>[4x]MGHHHHHHMSNEGLCAVCGDNAACQHYGVRTCEGCKGFFKRTVQKNAKYVCLANKNCPVDKRRRNRCQ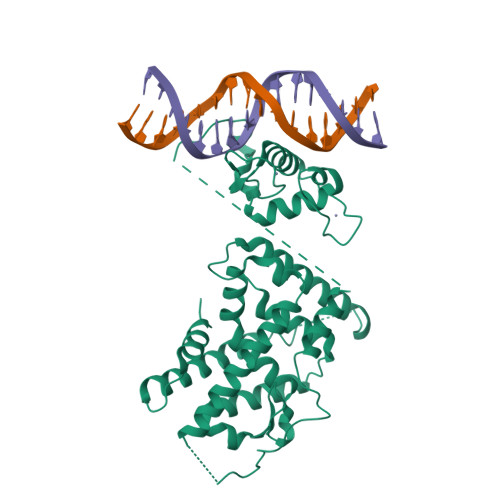YCRFQKCLAVGMVKEVVRTDSLKGRRGRLPSKPKSPQEPSPPSPPVSLISALVRAHVDSNPAMTSLDYSRFQANPDYQMSGDDTQHIQQFYDLLTGSMEIIRGWAEKIPGFADLPKADQDLLFESAFLELFVLRLAYRSNPVEGKLIFCNGVVLHRLQCVRGFGEWIDSIVEFSSNLQNMNIDISAFSCIAALAMVTERHGLKEPKRVEELQNKIVNCLKDHVTFNNGGLNRPNYLSKLLGKLPELRTLCTQGLQRIFYLKLEDLVPPPAIIDKLFLDTLPF>MKKVERFEVPRTIIFGPGALEKTPEVIPPSGRVLIITGKSSTRKYAERVAELLKQNCEIISYDQVELEKPGFDLVIGIGGGRPLDMAKVYSYIHKKPFVAIPTSASHDGIASPYVSFSLTQRFSKYGKISSSPVAIIADTSIILSAPSRLLKAGIGDLLGKIIAVRDWQLAHRLKGEEYSEYAAHLSLTSYKIAVGNAQKIKNFIREEDVRVLVKALIGCGVAMGIAGSSRPCSGSEHLFAHAIEVRVEKEDEVVHGELVALGTIIMAYLHGINWRRIKRIADIIGLPTSLRQANIDVDLALEALTTAHT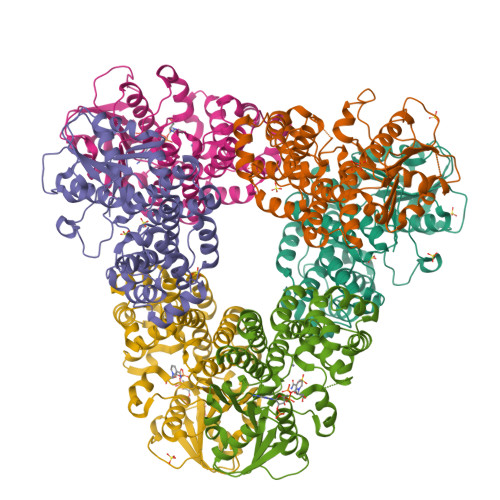LRPDRYTILGDGLSREAAKRALEDVELI[6x]> GSHMEAVQNRIVEAAERVPGVRGVIHLRARYVGQDIWADMIIGVDPENTVEQAHEICEAVQAAVCGKIRRIESLHVSAEAREI

One group of metal ion efflux transporters that regulates metal ion homeostasis and can be found in all domains of life is the Cation Diffusion Facilitator (CDF) protein family. One of the most highly conserved and abundant integral MM proteins is the CDF transporter MamM. MamM was recently proposed to function as a magnetosome-directed iron transporter required for iron biomineralization since its deletion abolished magnetite biomineralization and mutation of residues within the conserved TMD metal-binding site resulted in alterations of magnetite crystal size, morphology and even mineral phase. To summarize our results we present an alternative model for the CDF CTD mode of action, in which we propose that upon metal cation binding, the CTD induces conformational changes towards a tighter and more compact fold which allows the activation of iron transport through the TMD.

Each MamM monomer (residues 215–293) adopts the metallochaperone-like typical fold of CDF CTDs whilst the C-terminal tail (residues 294–318) is disordered and could not be traced in the electron density map. To validate that the disordered C-terminal tail have no effect on the domain fold, we determined the structures of a C-terminal truncation MamM-CTD mutant (residues 215–293) that adopted a similar CTD fold. As observed previously, the decreased number of particles per cell was at least partially a consequence of a substantial number of cells within the population that remained non-magnetic (10–20%). These previous studies also revealed that transcomplementation of a truncated C-terminal tail MamM mutant also allows the formation of wild-type-like particle. ITC measurements of the CTD single point mutants and the C-terminal truncation mutant revealed that the binding affinities remained in the same order of magnitude as the wild-type, with some alternation in the number of binding sites.> MLKKLFGAKKEFYVQLDESQAPAQVEEADVAIVKSEVAPVEKPAPTTSKKTSIKKKSATKA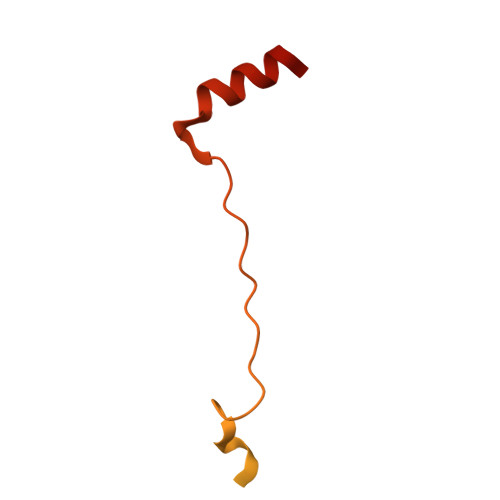AAPVETPASAPVAPAPKAKVDPSQVAFASGDPIPQNVARRTPGPSLNRFKEMARQVKVKR>EGDPIPEELYEMLSDHSIRSFDDLQRLLHGDPGEEDGAELDLNMTRSHSGGELESLARGRRSLGSLTIAEPAMIAECKTRTEVFEISRRLIDRTNANFLVWPPCVEVQRCSGCCNNRNVQCRPTQVQLRPVQVRKIEIVRKKPIFKKATVTLEDHLACKCETVAAHHHHHHH[2x];>LVVTPPGPELVLNVSSTFVLTCSGSAPVVWERMSQEPPQEMAKAQDGTFSSVLTLTNLTGLDTGEYFCTHNDSRGLETDERKRLYIFVPDPTVGFLPNDAEELFIFLTEITEITIPCRVTDPQLVVTLHEKKGDVALPVPYDHQRGFSGIFEDRSYICKTTIGDREVDSDAYYVYRLQVSSINVSVNAVQTVVRQG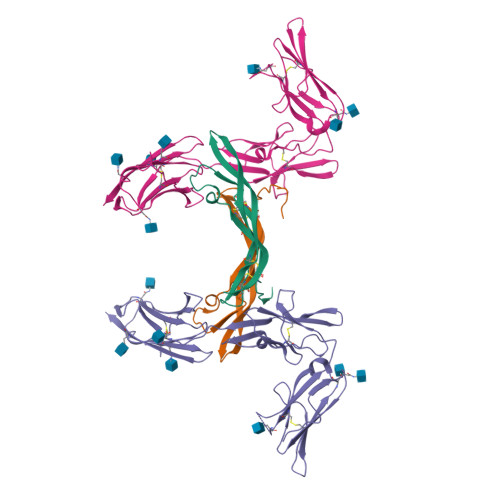ENITLMCIVIGNEVVNFEWTYPRKESGRLVEPVTDFLLDMPYHIRSILHIPSAELEDSGTYTCNVTESVNDHQDEKAINITVVESGHHHHHHH[2x]>MEKTDEYLLARFKGDGVKYKAKLIGIDDVPDARGDKMSQDSMMKLKGMAAAGRSQGQHKQRIWVNISLSGIKIIDEKTGVIEHEHPVNKISFIARDVTDNRAFGYVCGGEGQHQFFAIKTGQQAEPL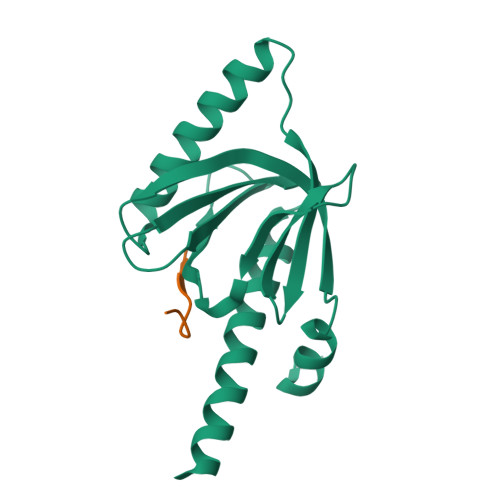VVDLKDLFQVIYNVKKKEEDKKKVEEANKAEEN[3x];>[3x]NGYENPTYK>[4x]DFLNPKYTLENFIVGEGNRLAYEVVKEALENLGSLYNPIFIYGSVGTGKTHLLQAAGNEAKKRGYRVIYSSADDFAQAMVEHLKKG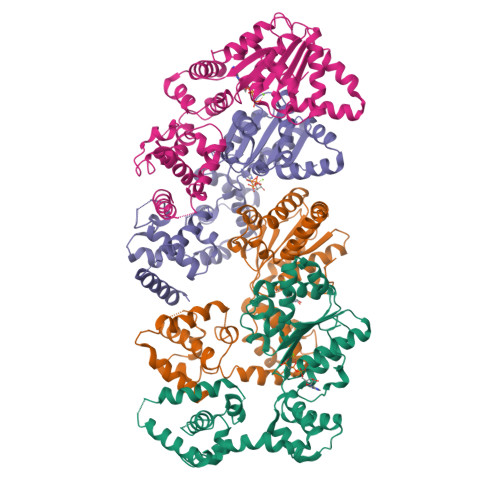TINEFRNMYKSVDLLLLDDVQFLSGKERTQIEFFHIFNTLYLLEKQIILASDRHPQKLDGVSDRLVSRFEGGILVEIELDNKTRFKIIKEKLKEFNLELRKEVIDYLLENTKNVREIEGKIKLIKLKGFEGLERKERKERDKLMQIVEFVANYYAVKVEDILSDKRNKRTSEARKIAMYLCRKVCSASLIEIARAFKRKDHTTVIHAIRSVEEEKKKDRKFKHLVGFLEKQAFDKIC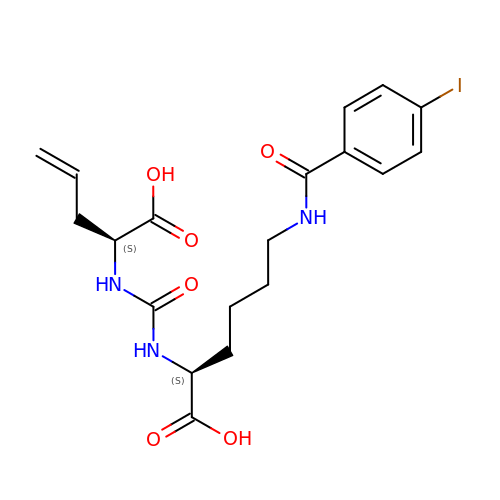N~2~-{[(1S)-1-carboxybut-3-en-1-yl]carbamoyl}-N~6~-[(4-iodophenyl)carbonyl]-L-lysine | C19 H24 I N3 O6 | CPITYBQMVPBERS-GJZGRUSLSA-N> XXXXXGSHMASMTGGQQMGRGSEFMRNELEEMQRRADQLADESLESTRRMLQLVEESKDAGIRTLVMLDEQGEQLDRVEEGMNHINQDMKEAEKNLK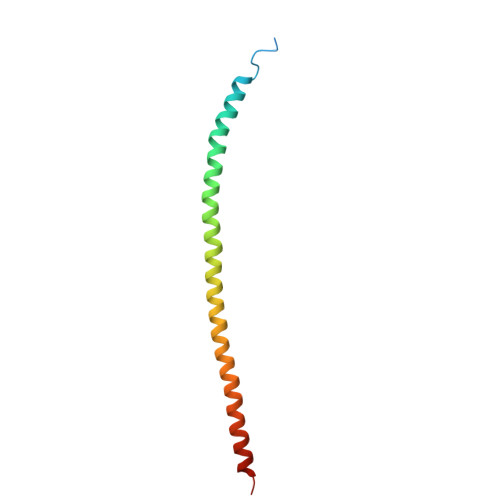DLG> MKFTVGNGQNQHKGVND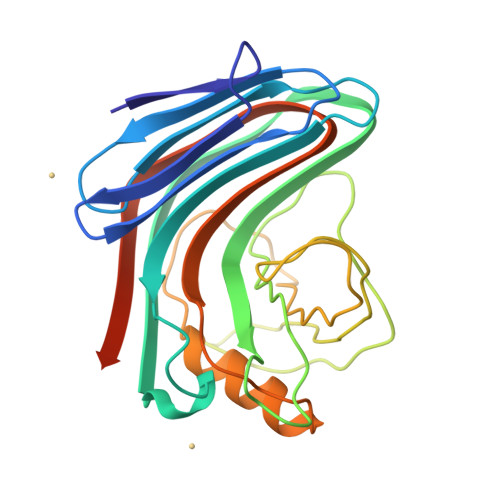GFSYEIWLDNTGGNGSMTLGSGATFKAEWNAAVNRGNFLARRGLDFGSQKKATDYDYIGLDYAATYKQTASASGNSRLCVYGWFQNRGLNGVPLVEYYIIEDWVDWVPDAQGKMVTIDGAQYKIFQMDHTGPTINGGSETFKQYFSVRQQKRTSGHITVSDHFKEWAKQGWGIGNLYEVALNAEGWQSSGVADVTLLDVYTTPKGSSPALEHHHHHH Aspartate/asparagine‐β‐hydroxylase (AspH) is a human 2‐oxoglutarate (2OG) and FeII oxygenase that catalyses C3 hydroxylations of aspartate/asparagine residues of epidermal growth factor‐like domains (EGFDs). Unusually, AspH employs two histidine residues to chelate FeII rather than the typical triad of two histidine and one glutamate/aspartate residue. AspH is highly unusual amongst structurally characterised 2OG dependent hydroxylases in employing only two residues, H679 and H725, to ligate its FeII. We report kinetic, inhibition, and crystallographic studies concerning human AspH variants in which either of its FeII binding histidine residues are substituted for alanine.

To investigate the structural basis of the kinetic differences between wt AspH and its variants, the latter were crystallised in the presence of MnII and 2OG or NOG, with or without the synthetic hFX‐EGFD186‐124‐4Ser substrate peptide. Similar results were obtained when H725A AspH was crystallised in the presence of MnII, 2OG, and hFX‐EGFD186‐124‐Ser, with a propionate ion being positioned to interact with R735 and S668, though the propionate was observed in two conformations. The crystallographic studies also unambiguously reveal the presence of only one potential FeII‐binding histidine residue for the H679A and H725A AspH variants. Unexpectedly, the results revealed that, whilst the variants were less active than wt AspH, they both retained substantial activity: in particular the H679A variant manifested ≈50 % substrate turnover under conditions where wt AspH gave >95 % turnover (30 minutes incubation); the H725A variant was less active (<5 %), but clear evidence for substrate hydroxylation was observed by mass spectrometry (MS). By contrast, the kcatapp ‐values for the H725A AspH variant are approximately half those for H679A AspH, in agreement with the observed lower substrate hydroxylation in our initial turnover assays. The H725A AspH substitution appears to have a more pronounced effect than the H679A substitution on the Kmapp ‐values for FeII, which are approximately twofold and threefold higher than those of wt and H679A AspH, respectively (entries 1 and 2). Strikingly, for H725A AspH, the Kmapp ‐value for 2OG is ≈200 times greater than that of wt AspH and about double that of H679A AspH (entry 3). By contrast, the H725A AspH Km ‐value for the hFX‐EGFD186‐124‐4Ser substrate peptide is in the range of that of H679A AspH (entry 4). The H725 imidazole that coordinates FeII opposite to the proposed O2‐coordination site may similarly regulate the stability of O2 (and 2OG) derived intermediates, including the FeIII‐2OG‐superoxide species in catalysis.

> KPKLLNKFDKTIKAELDAAEKLRKRGKIEEAVNAFKELVRKYPQSPRARYGKAQCEDDLAEKRRSNEVLRGAIETYQEVASLPDVPADLLKLSLKRRSDRQQFLGHMRGSLLTLQRLVQLFPNDTSLKNDLGVGYLLIGDNDNAKKVYEEVLSVTPNDGFAKVHYGFILKAQNKIAESIPYLKEGIESGDPGTDDGRFYFHLGDAMQRVGNKEAYKWYELGHKRGHFASVWQRSLYNVNGLKAQPWWTPKETGYTELVKSLERNWKLIRDEGLAVMDKAKGLFLPEDENLREKGDWSQFTLWQQGRRNENACKGAPKTCTLLEKFPETTGCRRGQIKYSIMHPGTHVWPHTGPTNCRLRMHLGLVIPKEGCKIRCANETKTWEEGKVLIFDDSFEAEVWQDASSFRLIFIVDVWHPELTPQQRRSLPAI;> DGDQSETSPSQNQGKCKDGLGEYTCTSLEGFEGKNSELF> GSLSNTIQQKILKLPDKYRTVIVLKYIDELSLIEIGEILNIPVGTVKTRIHRGREALRKQLR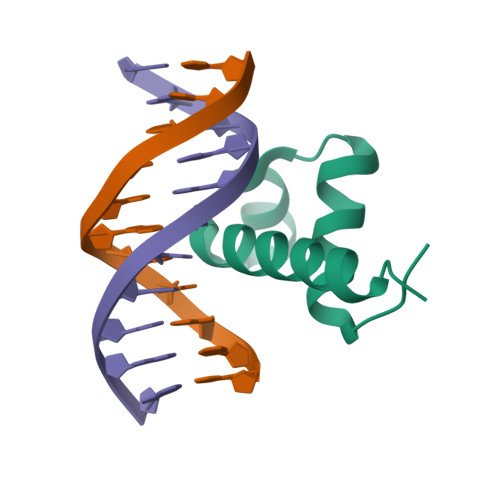DL>[7x]AMADIGSEFDDNDVATAKATGETSAKVSINKVLNIAEGIT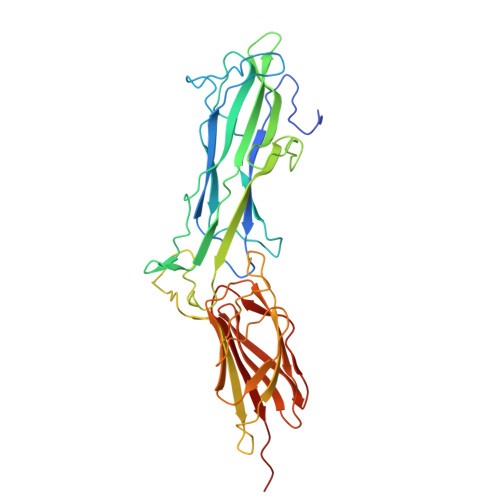TPEATFTFTFTPKTGTSSNGAPYETIDSSNGQITDKNVSYSGTDVLATGQTNIKKDTGDIFREVNYTHAGEYVYTVAEKQNVGWKVIQKNGSPIDFMTYDNRNYEMHVIVKNKTTGGTYISSVYFKQVSPSVNGKVKPSESGTTYKYDLFTNIYRKNAGKITDPNEPNPNKPNVSKVDPNAKSLVIKKVVSGATADKSKDFTFKLTFTKASTETSQSITGKIGETSKTFVYGQETTITLRHDQSLVFDTIPAGTRYKLVETGSQGYTASAAYKENGASKNQAGTVSTNFTQDSILIGEKPNDNTITNSLPDVTPT> HMMGGISICVATDCDGEKVNLRFLFDAAGPSVSRLLNYSTTAFNNYFRLKGISRAFAVNS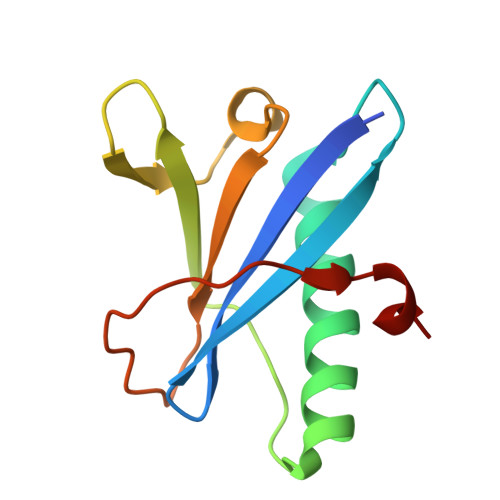AVVFNDVHCTWDRLERTTQLLHNSQVYLFQPDTLDIPAAIPEPYEGEPLLSA The Yersinia outer protein J (YopJ) family effectors are widely deployed through the type III secretion system by both plant and animal pathogens. As non-canonical acetyltransferases, the enzymatic activities of YopJ family effectors are allosterically activated by the eukaryote-specific ligand inositol hexaphosphate (InsP6). Among them, PopP2 produced by the root-infecting bacterium R. solanacearum acetylates a conserved lysine residue in WRKY transcription factors to inhibit the expression of defense-related genes. Our recent studies identified a previously undescribed regulatory domain in the structures of PopP2 and HopZ1a. Both the binding pockets of InsP6 and the acetyl group donor acetyl-coenzyme A (AcCoA) are located on the interface between the regulatory domain and the catalytic core.

To understand how InsP6-binding induces the structural change of YopJ effectors, we crystallized the entire acetyltransferase domain (residues 149–488) of PopP2 in the absence of InsP6. The apo-state PopP2 structural model consists of a five-stranded β-sheet sandwiched by αD, αE, and αF from one side and αC from the other side and a helix-bundle formed by the αB and αA from the very N-terminus and αG and αH from the very C-terminus. The catalytic triad, including His260, Asp279, and Cys321 residues, are well preserved in the structure. On the other hand, the entire regulatory domain (residues 377–447) was unable to build due to its missing electron density. Structural comparison of the apo-PopP2 structure with that of the InsP6-bound PopP2 reveals that the catalytic core is well conserved, giving a root mean square deviation (RMSD) of 0.5 Å over the Cα atom of 248 aligned residues. The most striking difference lies in a segment ahead of the N-terminus of the regulatory domain (residues 351–375), which is able to adopt two entirely different structures with distinct sets of packing interactions. In the apo conformation, this segment exists as a long α-helix (αF) that is packed against αE and β5 mainly through hydrogen bonds and hydrophobic interactions; by contrast, in the PopP2-InsP6 complex structure, the same set of residues are folded into two antiparallel β-strands (β6’ and β7’) linked by a long loop (Lβ6’β7’). Indeed, it is apparent that αF in apo-PopP2 would sterically clash with the first helix of the regulatory domain, which harbors R380 and K383 residues that directly interact with the phosphate groups of InsP6. In the apo structure, only a short loop (Lβ4β5) containing residues 296–302 was built with poor electron density. The C-terminus of αG is too close to the Lβ8’β9’ of the regulatory domain and RRS1WRKY in the overlapped structures, suggesting that the stabilization of the regulatory domain by InsP6 leads to disruption of the C-terminal helical structure of αG to save room for substrate binding.

> GRQAGQQATVGRLRTQVTGFLSGALGKLQALSAQNMDPELAQFRVLDVDRAIMPLLIVAENARNPGLNLVPLHMDMAEDEEVRTQPPMAGSRHIAEFVASARPGRYRAVIDDGSHTRAADIRKDASGTSVIVVDPLRKEKDESAYVDYADNVNMEFGEHAKCAFIPVDIQKSFFDCRILSLSLALKMHDKDDAFAAFHETLRNGGDPSHHVSRAQQTEELGATLVLDGAPLVDARMMKHGQAASSVSRYLGNHPEQSTVPVNKRNETLGERTTRHLVKRKVRNRADSEGRVTSGETKEITFSNSVEQKRIALLNRAASYVNSAPPPVVMRMAKLLQDSLLDTN>[2x]GSHMTDSMNTLVTPLQRSDAPQLEPVFRGMEQ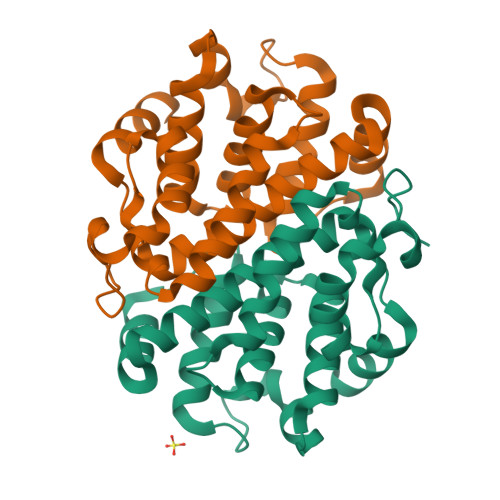NLGFLPNGILTMGKNPDLAVAFGGLFKCIDAFKHIPTELKWAIAMISSSAAGCMYCKSHFSHIATRTHVNRNKVMAAFEFQTSDFYNEAERAALAFAFANSTSPAHLDKEHFDELARYYSEEAAIEIAAIIAICGFLNRWNAAMDSQIEAAPRATLDEIEKQN> SMAILFAVVARGTTILAKHAWCGGNFLEVTEQILAKIPSENNKLTYSHGNYLFHYICQDRIVYLCITDDDFERSRAF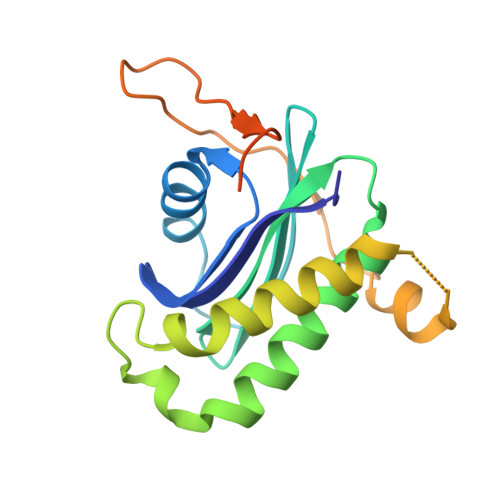SFLNEVKKRFQTTYGSRAQTALPYAMNSEFSSVLAAQLKHHSENKSLDKVMETQAQVDELKGIMVRNIDLVAQRGERLELLIDKTENLVDSSVTFKTTSRNLARAMCMKNIK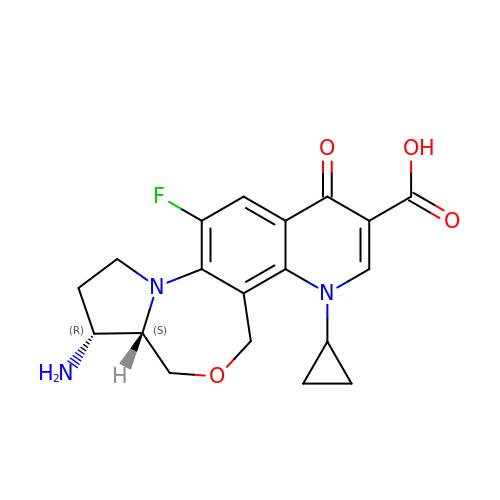(3aS,4R)-4-amino-13-cyclopropyl-8-fluoro-10-oxo-3a,4,5,6,10,13-hexahydro-1H,3H-pyrrolo[2',1':3,4][1,4]oxazepino[5,6-h]quinoline-11-carboxylic acid | C19 H20 F N3 O4 | DXDXKLSOWWPCNV-HUUCEWRRSA-N> SRAFQPEFVESISNVSVAVGRDATFTCHVRHLGGYRVGWLKADTKAIQAIHENVITHNPRVTVSHLDQNTWN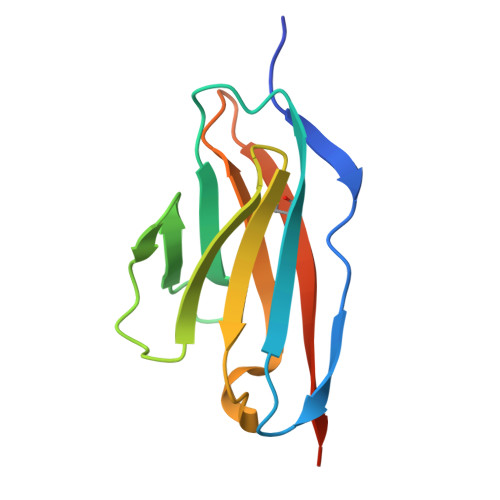LHIKAVSEEDRGGYMCQLNTDPMKSQIGFLDVVIPHHHHHH>SNAMAPPPFRPENAIKRADELISVGEKQAALQSLHDFITARRIRWATPSTVEPVVFKFLEIGVELKKGKLLKDGLHQYKKLIQGSTEGLVSVGAVARKFIDLVESKIASEQTRADELQKQEIDDDLEGGVTPENLLISVYESDQSVAGFNDEAITSWLRFTWESYRAVLDLLRNNALLEITYSGVVKKTMHFCLKYQRKNEFKRLAEMLRQHLDAANYQQSKSGNNLVDLSDADTLQRYLDQRFQQVDVSVKLELWHEAYRSIEDVFHLMKISKRAPKPSTLANYYENLVKVFFVSGDPLLHTTAWKKFYKLYSTNPRATEEEFKTYSSTIFLSAISTQLDEIPSIGYDPHLRMYRLLNLDAKPTRKEMLQSIIEDESIYGKVDEELKELYDIIEVNFDVDTVKQQLENLLVKLSS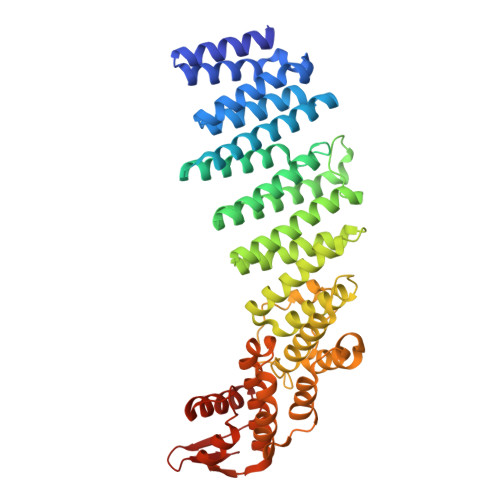KTYFSQYIAPLRDVIMRRVFVAASQKFTTVSQSELYKLATLPAPLDLSAWDIEKSLLQAAVEDYVSITIDHESAKVTFAKD[3x]>[2x]MHHHHHHGEASPVDPLRPVVDASIQPLLKEHRIPGMAVAVLKDGKAHYFNYGV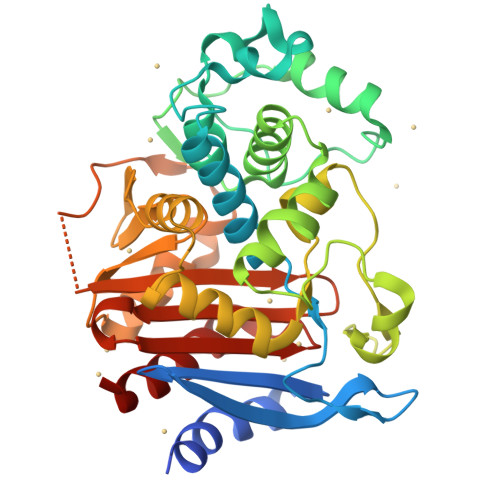ANRESGAGVSEQTLFEIGSVSKTLTATLGAYAVVKGAMQLDDKASRHAPWLKGSAFDSITMGELATYSAGGLPLQFPEEVDSSEKMRAYYRQWAPVYSPGSHRQYSNPSIGLFGHLAASSLKQPFAPLMEQTLLPGLGMHHTYVNVPKQAMASYAYGYSKEDKPIRVNPGMLADEAYGIKTSSADLLRFVKANIGGVDDKALQQAISLTHQGHYSVGGMTQGLGWESYAYPVTEQTLLAGNSAKVILEANPTAAPRESGSQVLFNKTGSTNGFGAYVAFVPARGIGIVMLANRNYPIEARIKAAHAILAQLAG>[2x]MHHHHHHSSGRENLYFQGHMDRLITLVVSYSIAFSIFALATMAVVYGKWLYYFEIDFLNIPDLADMTKDEIKRNYDVLITYLSPFYDGALHLPTLDMSTNGRIHFVDVKNILVKIQYVMYA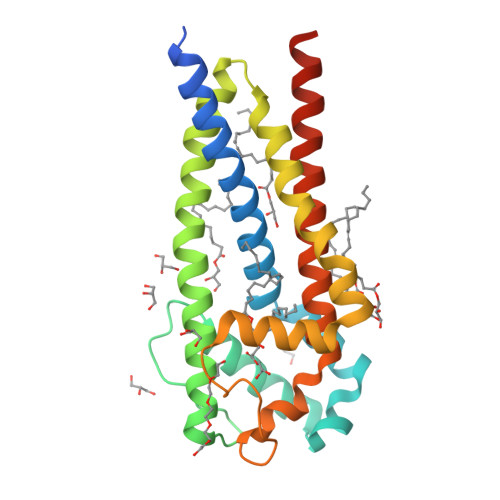TIMIAVIGGIYLLKKKNEKFLLHGSILTIIFPIALMLPIAINFEKSFVLFHKLLFSNDYWVFDPEKDPIILMLPEEFFMHAACAILLFILGGSILCYSLYRYLVKKKRMSQKKFSA>MLYNVALIKFKDIADKRGHLTPIEGKIDIPFDIKRVYYITKVDKDITRGYHSHK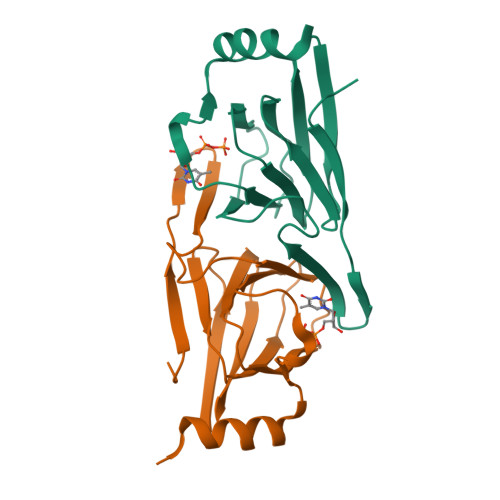KLHQVLICLNGSVKIRLKIPDEEKIIELNDPSVGLYIGPLVWHEMFDFTEGCVLLVLASEYYDETDYIRNYDFYIDEAKKRFLEHHHHHH[8x]> MKTEFSGDTDAVHGKTHVFIRSIKNGSHMQEAKIDIKSLYDSLAKKYDVQHKNSYEVIYPKGYEIKVLGNKYVKLVAMSRHKTQKHLVKIVVKSEKTIDSLDPIRQKSLLKKQDEVVVTTDHIAMVYNDDHFFENVNAKNLKVGNYVSVYDEASDKEVIGEIASIEDLGMTDDYVYDAEVDDDSHAFYASNILVHASQFCNGTKLGG

Here, we report the novel and atypically split PolB16 OarG intein and its biochemical and structural characterization. The PolB16 intein carries an atypical split position close to the N-terminal end of the encoded split intein domain to give IntN and IntC fragments of 15 and 168 aa, respectively. Most notably, both residues at the 1 and +1 positions are serine. Furthermore, the intein overall exhibits the typical conserved motifs of a class 1 intein29 that represent conserved residues across inteins, of which some are involved in catalyzing the steps of the protein splicing pathway. This analysis suggested the PolB16 intein splices through linear and branched oxoester intermediates.

The IntC fragment contains two cysteines within motifs N3 and C2,30 (previously also referred to as motifs B and F)31 however, at non-essential and only moderately conserved positions that usually harbor hydrophobic residues. By replacement of two non-conserved cysteines, it could be mutated into a completely cysteine-less variant and further engineered for efficient splicing properties. To this end, we genetically fused the IntN and IntC precursors, each with 10 extein residues, with a 3 amino acid linker (GSH). Ser1 and Asn183 at the splice junctions were mutated to alanine to block all splicing activity. We obtained protein crystals in this format for both the wild-type sequence and the cysteine-less double mutant (C111A, C165A) and could solve these at resolutions of 1.85 and 2.6 Å, respectively. Both structures were virtually identical (0.185 Å RMSD, root mean square deviation), consistent with the negligible functional impact of mutating the non-conserved cysteine residues (Fig. S6†). The last well-resolved amino acids, Asp108 and His109, show a conformation of the polypeptide chain that departs from the canonical intein structure. As a consequence, His109 is placed in an unusual position, remote from the scissile bond (Fig. 6 and S7C†), which is incompatible with its usual catalytic role. Our PolB16 intein structures showed the motif NX histidine in possible hydrogen-bond forming distance to the Ser1, when the side chain hydroxyl of the latter is modeled back in (3.0 Å).>MAGYLNNIALNLEIVLKNKADSPEVSETLVTRICENLLLSKEVSFL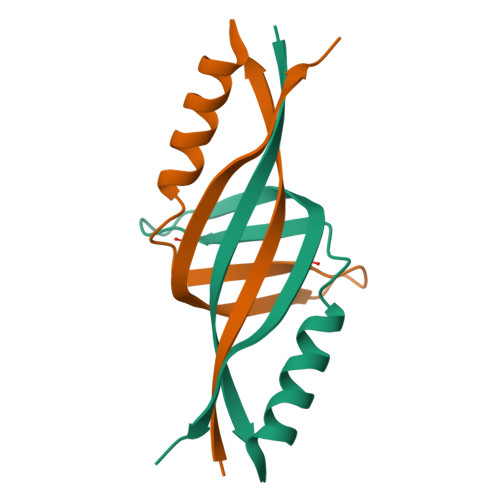KADGSVENFKLSDMEYEITNTEELPELEHHHHHH[2x]>[84x]MGLFDRIKRVVSSNLNDLVNKAEDPEKMLEQAILEMQEDLVQLRQGVAQAIAAQKRSEKQYNDAQNEINKWQRNAQLALQKGDENLARQALERKKTYTDTSAALKASLDTQSTQVETLKRNLIQLESKISEAKTKKEMLKARITTAKAQEQLQGMVRGMNTSSAMSAFERMEEKVLMQESRAQALGELAGADLETQF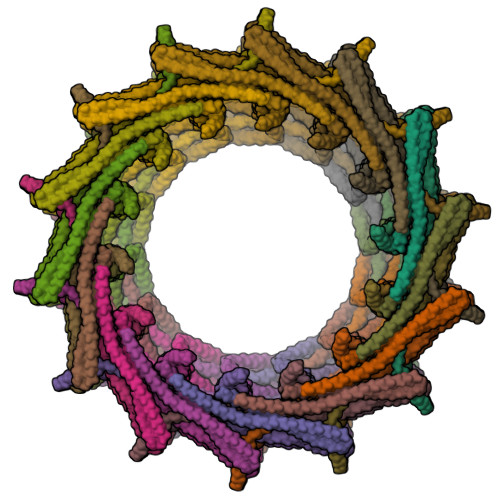AQLEGGSDVDDELAALKAQMLPPATPVTQAQLPPQQETTPAKSNEVVDAELDSLRKQLDQL> RMVDLPVIQPRLCTHARWPAPVYGLLVDPSLPSNPQWQNGRVHVDGTLLGTTPISGSWVSCFAAEAAYKFQSGTGEVATFTLIEQDGSAYVPGDRAAPLGYPDFSGQLEIEVQTETTKT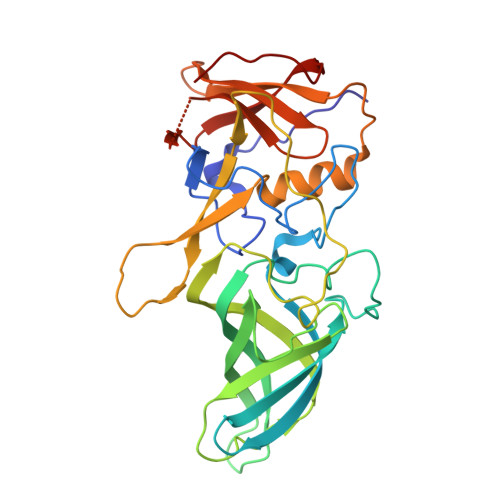GDKLKVTTFEMILGPTTNADQAPYQGRVFASVTAAASLDLVDGRVRAVPRSIYGFQDTIPEYNDGLLVPLAPPIGPFLPGEVLLRFRTYMRQIDTADAAAEAIDCALPQEFVSWFASNAFTVQSEALLLRYRNTLTGQLLFECKLYNEGYIALSYSGSGPLTFPTDGIFEVVSWVPRLYQLASV~{N}-[3,3,3-tris(fluoranyl)propyl]benzamide | C10 H10 F3 N O | 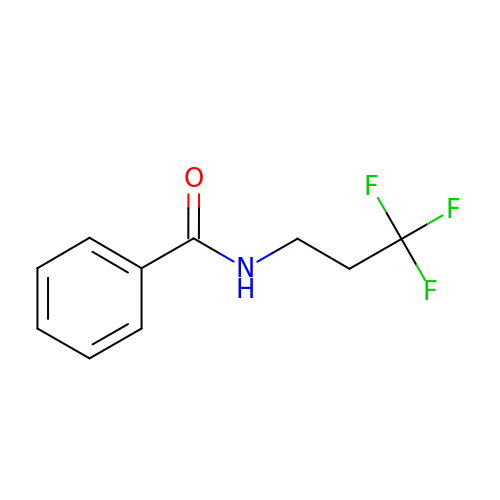HGTGCLBXLPLRNB-UHFFFAOYSA-N8-amino-N-hydroxyoctanamide 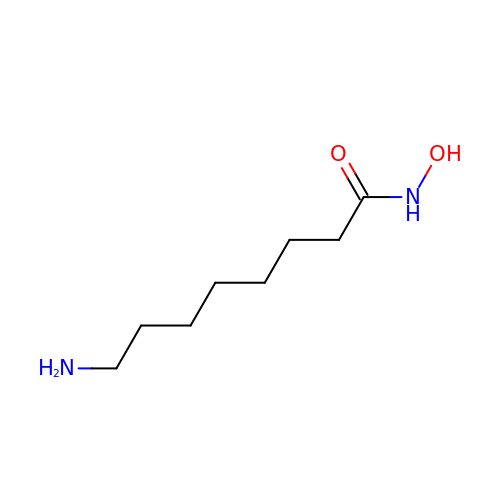| C8 H18 N2 O2 | GPJAXDUQXFPTEI-UHFFFAOYSA-N>MRINHNIAALNTSRQLNAGSNAASKNMEKLSSGLRINRAGDDAAGLAISEKMRSQIRGLDMASKNAQDGISLIQTSEGALNETHSILQRMSELATQAANDTNTDSDRSELQKEMDQLASEVTRISTDTEFNTKKLLDGTAQNLTFQIGANEGQTMSLSINKMDSESLKVGTTYTANDDGSKLVTADGKEATLVTDGSKGPNGYYDDADKLVYQADSALAKDTKVTKGIDISSSAKAASSALTTIKTAIDTVSSERAKLGAVQNRLEHTINNLGTSSENLTSAESRIRDVDM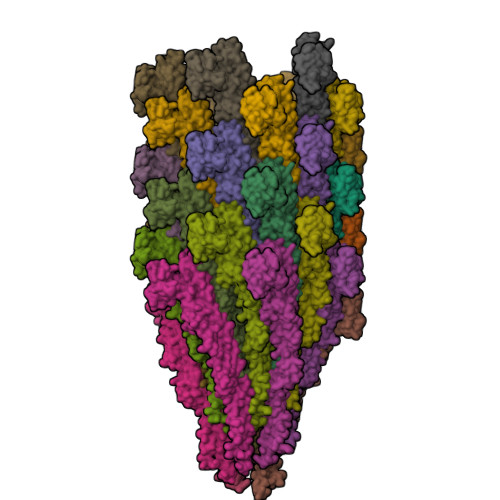ASEMMEYTKNNILTQASQAMLAQANQQPQQVLQLLKG[33x]>MLSATQPLSEKLDSTLKHLAIIMDGNGRWAKLKNKARAYGHKKGVKTLKDITIWCANHKLECLTLYAFSTENWKRPKSEVDFLMKMLKKYLKDERSTYLDNNIRFRAIGDLEGFSKELRDTILQLENDTRHFKDFTQVLALNYGSKNELSRAFKSLLESPPSNISLLESLENEISNRLDTRNLPEVDLLLRTGGEMRLSNFLLWQSSYAELFFTPILWPDFTPKD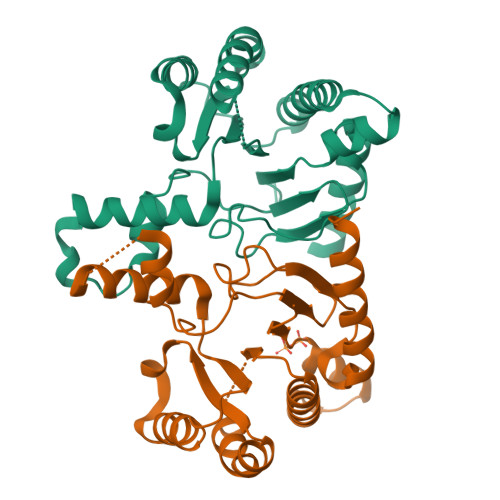LENIISDFYKRVRKFGELKA[2x]>GSHMSEELNNGENSLLKNLEDGFTIWLTGPSGAGKSTLAYALEKKLLEKGFRVEILDGDVIRNTLYPNIGFSKEAREMHNRVVIHLAKLLSKNGVITIVSLISPYRAVREYARKEIQNFMEVYIHSPLEVRIQRDPKGLYAKALKGEIKGLTGYDGVYEEPENPELKIESHKMSIEEEVDTVIRTAQKLGYL[4x]

Methanothermococcus thermolithotrophicus is the only known methanogen that grows on sulfate as its sole sulfur source, uniquely uniting methanogenesis and sulfate reduction. Here we use physiological, biochemical and structural analyses to provide a snapshot of the complete sulfate reduction pathway of this methanogenic archaeon. M. thermolithotrophicus activates SO42− by conventional ATPS and APSK, but transforms it further by uncanonical enzymes.

(1b) Alternatively, APS can be further phosphorylated to 3′-phosphoadenosine 5′-phosphosulfate (PAPS) by the APS kinase (APSK). The APS-kinase model from M. thermolithotrophicus, MtAPSK, was refined to 1.77 Å. MtAPSK forms a homodimer with an organization very similar to bacterial enzymes, which was expected due to its high sequence conservation. Despite co-crystallization and soaking the crystals with APS and MgCl2, the MtAPSK structure was obtained in its apo state with a bound phosphate at the expected position of the ATP β-phosphate. The N terminus and region 125–152 (the latter being involved in substrate binding) could not be modelled due to the lack of electron density. However, the residues binding the substrates and Mg2+ are conserved, suggesting that MtAPSK should be functional, as confirmed by the coupled enzyme assay. The activity of the recombinantly expressed MtATPS and MtAPSK was tested via a coupled assay and a specific activity of 0.070 ± 0.004 µmol of oxidized NADH min−1 mg−1 of MtATPS was measured.>[4x]AEAGITGTWYAQLGSTFIVTAGADGALTGTYESAVGNAESRYVLTGRYDSAPATDGSGTALGWTVAWKNNYRNAHSATTWSGQYVGGAEARINTQWLLTSGTTEANAWKSTL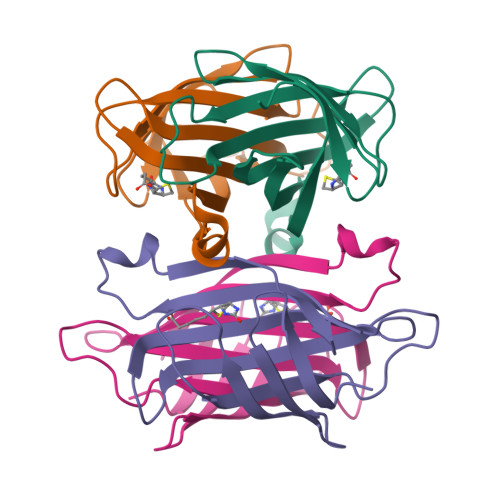VGHDTFTKVKPSAAS> MAGLASLSSVGALRGMRLVPAAHLLPLHSAFGQQTRNFGAGDLKIVAARMKSVKSIQKITKAMKMVAASKLRMDQRRLENGLPFATPVQKLVQRIPVDPKEKGTLAVLALSSDKG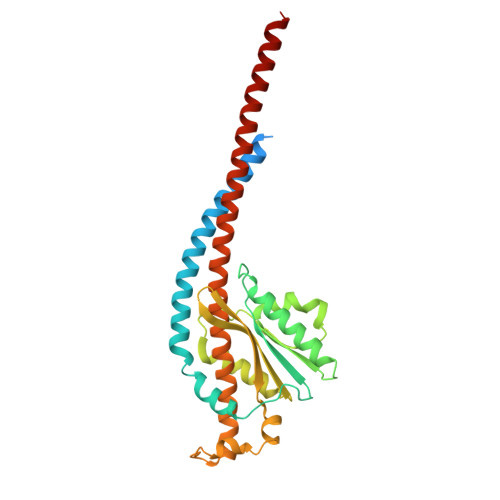LCGGVNSFVAKQARIVIKENEMAGNAVQVYGVGDKIRSALQRTFGDRFKRIMTEVTRFPWNFGQACIIADRLMQDNPARLMVIYNHFKSAVAYDTLTLNVLTPTQAAQSAKEQLNTFEFEPEKTDVWKDLQDFYYACTVFGCMLDNIASEQSARMSAMDNASTNAGEMISSLTLRYNRARQAKITTELVEIISGANALE>[2x]S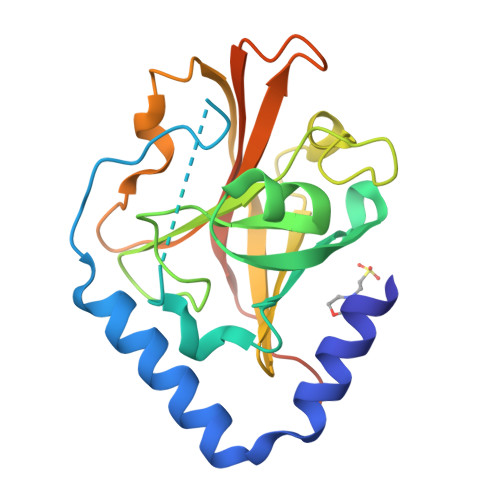NEVIKEFDETVSQMDKAELEERWRLAQAFNATLKPSEILDPFTEQEKKKGVSEYANMLKVHERIGYVEIPAIDQEIPMYVGTSEDILQKGAGLLEGASLPVGGENTHTVITAHRGLPTAELFSQLDKMKKGDIFYLHVLDQVLAYQVDQIVTVEPNDFEPVLIQHGEDYATLLTCTPYMINSHRLLVRGKRIPYTAPIAERNRAVRERGQF> SHQAPVIPDDFRCPISLELMKDPVIVSTGQTYERTCIEKWLQAGHGTCPKTQQTLTSTVLTPNYVLRSLIAQ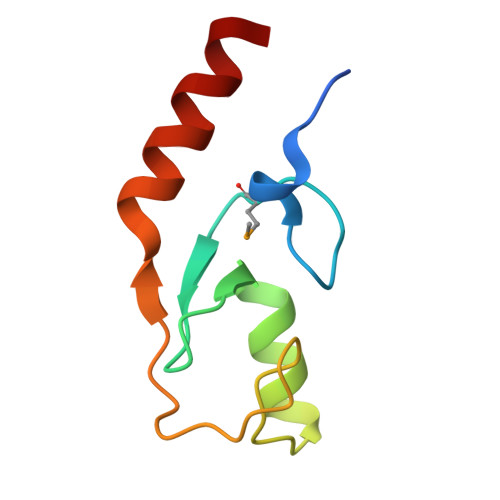WCEAN> MSLILLGALSLASSTFAQTWIWYPGDYEIWLGNQMNNRRTERGAFFPPFWKTDSHYVVVEFSKVLNLSEPEEVFIAAEGTYNVKLDGKLQFGMPETLLLPAGKHSLNIKVWNQATPPTIYVKGKTVNSDSSWRVTYEDKEWIDESGKASDTSATIYMDAGCWNFDGATQRPSQFSLMREPQQPVAKTEQPEGGILYDFGKETFGFITLKNLSGKGKIDLYYGESPEEAKDKAYCETLDKLLLEPGQITDLAIRSTSPLHHSDNEYTLENSKAFRYVYITHEPEVQIGEVSMQYEYLPEEYRGNFRCNDEELNCIWEVGAYTMHLTTREF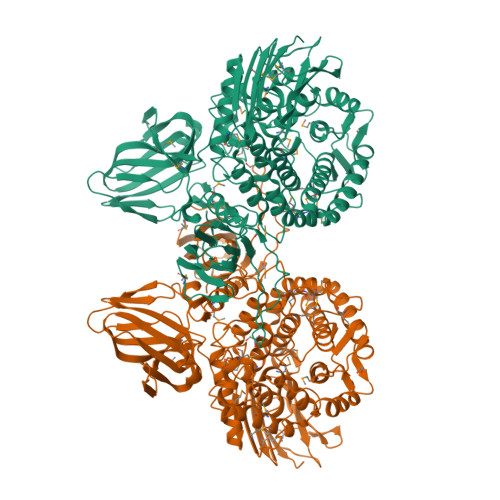FIDGIKRDRWVWSGDAIQSYLMNYYLFFDSESVKRTIWLLRGKDPVTSHSNTIMDYTFYWFLSVYDYYMYSGDRHFVNQLYPRMQTMMDYVLGRTNKNGMVEGMSGDWVFVDWADGYLDKKGELSFEQVLFCRSLETMALCADLVGDKDGQQKYEKLASALKAKLEPTFWNNQKQAFVHNCVDGRQSDAVTRYANMFSVFFDYLNADKQQAIKQSVLLNDEILKITTPYMRFYELEALCALGEQETVMKEMKAYWGGMLKAGATSFWEKYNPEESGTQHLAMYGRPYGKSLCHAWGASPIYLLGKYYLGVKPTKEGYKEFAVSPVLGGLKWMEGTVPTPNGDIHVYMDNKTIKVKATEGKGYLTIQSRRQPKANMGTVEKVSEGVWRLWIDSPEERIVTYRLEGHHHHHH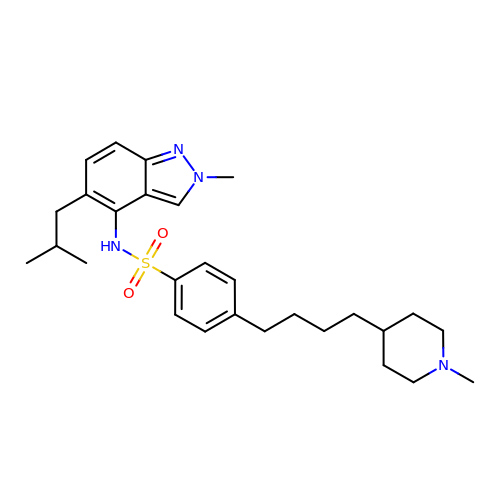~{N}-[2-methyl-5-(2-methylpropyl)indazol-4-yl]-4-[4-(1-methylpiperidin-4-yl)butyl]benzenesulfonamide | C28 H40 N4 O2 S | HAEBJCXYCZWIGA-UHFFFAOYSA-N>[2x]MSSQKVFGITGPVSTVGATAAENKLNDSLIQELKKEGSFETEQET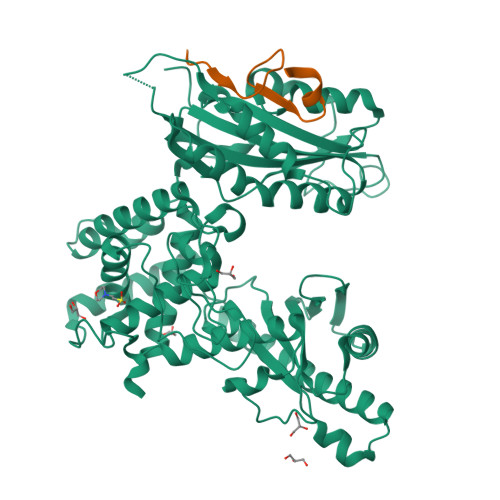ANRVQVLKILQELAQRFVYEVSKKKNMSDGMARDAGGKIFTYGSYRLGVHGPGSDIDTLVVVPKHVTREDFFTVFDSLLRERKELDEIAPVPDAFVPIIKIKFSGISIDLICARLDQPQVPLSLTLSDKNLLRNLDEKDLRALNGTRVTDEILELVPKPNVFRIALRAIKLWAQRRAVYANIFGFPGGVAWAMLVARICQLYPNACSAVILNRFFIILSEWNWPQPVILKPIEDGPLQVRVWNPKIYAQDRSHRMPVITPAYPSMCATHNITESTKKVILQEFVRGVQITNDIFSNKKSWANLFEKNDFFFRYKFYLEITAYTRGSDEQHLKWSGLVESKVRLLVMKLEVLAGIKIAHPFTKPFESSYCCPTEDDYEMIQDKYGSHKTETALNALKLVTDENKEEESIKDAPKAYLSTMYIGLDFNIENKKEKVDIHIPCTEFVNLCRSFNEDYGDHKVFNLALRFVKGYDLPDEVFDENEKRPSKKSKRKN;>[2x]DLEVIISLGPDPTRLDAKLLDSYSTA>EELPAPVKAIEKQGITIIKTFDAPGGMKGYLGKYQDMGVTIYLTPDGKHAISGYMYNEKGENLSNTLIEKEIYAPAGREMWQRMEQSHWLLDGKKDAPVIVYVFADPFCPYCKQFWQQARPWVDSGKVQLRTLLVGVIKPESPATAAAILA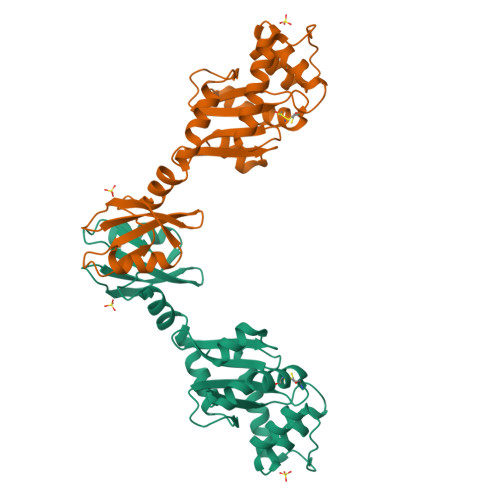SKDPAKTWQQYEASGGKLKLNVPANVSTEQMKVLSDNEKLMDDLGANVTPAIYYMSKENTLQQAVGLPDQKTLNIIMGNKLQHHHHHHHH[2x]6-[(3~{R})-3-oxidanylpyrrolidin-1-yl]-5-pyrimidin-5-yl-~{N}-[4-(trifluoromethyloxy)phenyl]pyridine-3-carboxamide 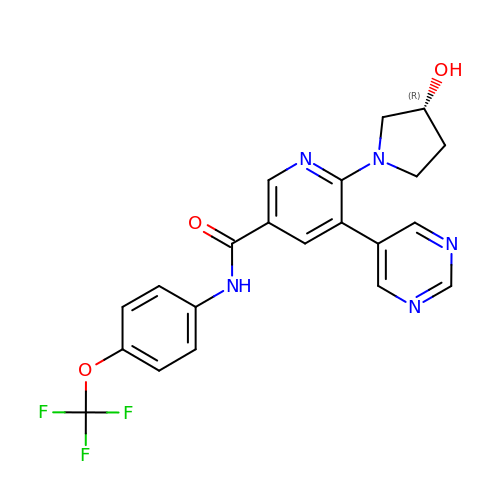| C21 H18 F3 N5 O3 | LARFZNXVNANWFD-MRXNPFEDSA-N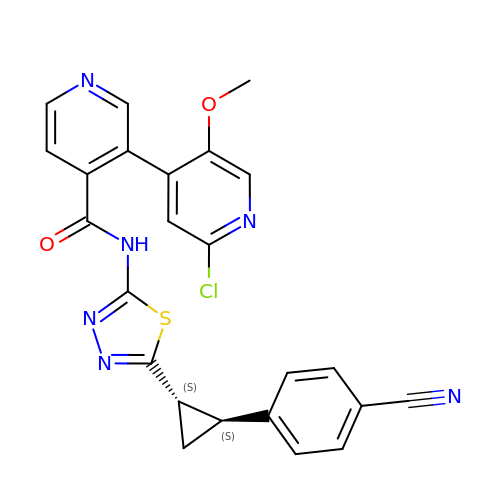(3M)-2'-chloro-N-{5-[(1S,2S)-2-(4-cyanophenyl)cyclopropyl]-1,3,4-thiadiazol-2-yl}-5'-methoxy[3,4'-bipyridine]-4-carboxamide | C24 H17 Cl N6 O2 S | NNLVUZZKRCTPAP-AEFFLSMTSA-N>AASGLEAAMKAAGKQYFGTALTVRNDQGEIDIINNKNEIGSITPENAMKWEAIQPNRGQFNWGPADQHAAAATSRGYELRCHTLVWHSQLPSWVANGNWNNQTLQAVMRDHINAVMGRYRGKCTHWDVVNEALNEDGTYRDSVFLRV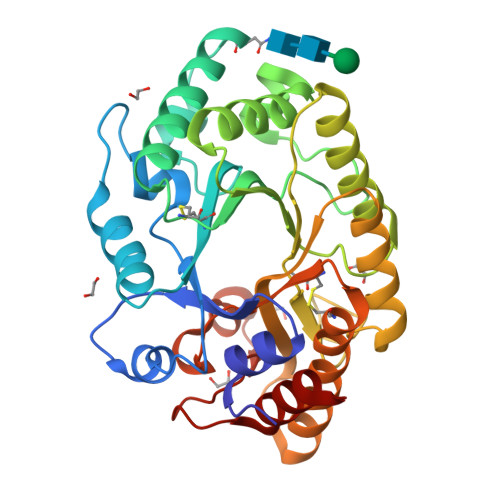IGEAYIPIAFRMALAADPTTKLYYNDYNLEYGNAKTEGAKRIARLVKSYGLRIDGIGLQAHMTSESTPTQNTPTPSRAKLASVLQGLADLGVDVAYTELDIRMNTPATQQKLQTNADAYARIVGSCMDVKRCVGITVWGISDKYSWVPGTFPGEGSALLWNDNFQKKPSYTSTLNTINRR[5x]>SNAMFAPQGLAQFIKVNVTLENGEPVFIYTDANGQVCQGDITVTQAGTITYLLNDQTLKGLKFVGVGFVTPFDG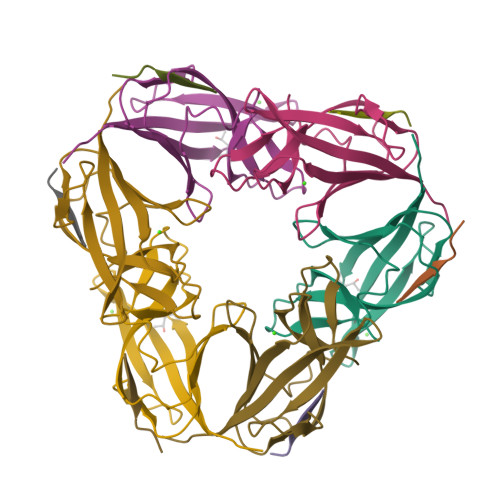IIDAVTISSDGMLVQLVDLDKTPGTTKFQFVLSNTANTLLVLSPD[2x];>[2x]PAIINRPQN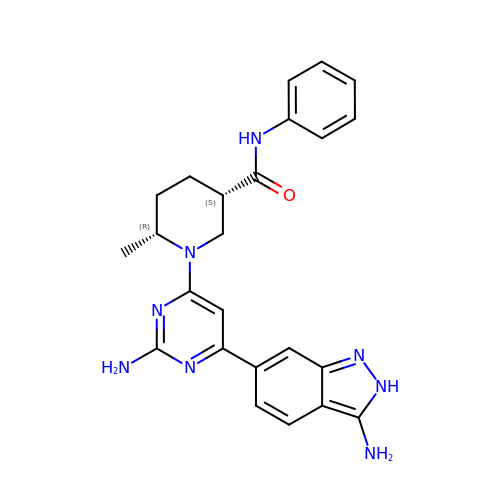(3S,6R)-1-[2-amino-6-(3-amino-2H-indazol-6-yl)pyrimidin-4-yl]-6-methyl-N-phenylpiperidine-3-carboxamide | C24 H26 N8 O | TXXYVBLFLGPQOR-ZBFHGGJFSA-N(8R)-3-beta-D-ribofuranosyl-3,6,7,8-tetrahydroimidazo[4,5-d][1,3]diazepin-8-ol 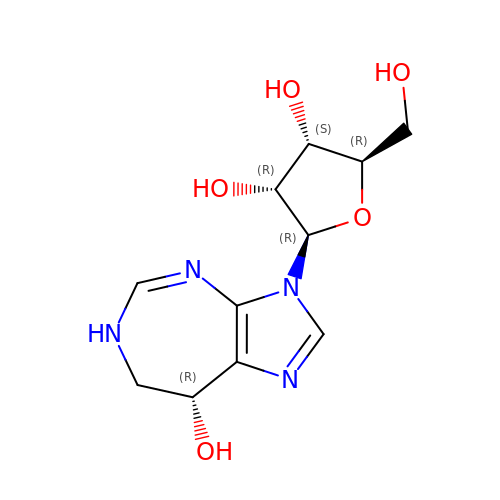| C11 H16 N4 O5 | YOOVTUPUBVHMPG-LODYRLCVSA-N> SMGESRVILAFGDSLFAGYGLDKGESYPAKLETALRSHGI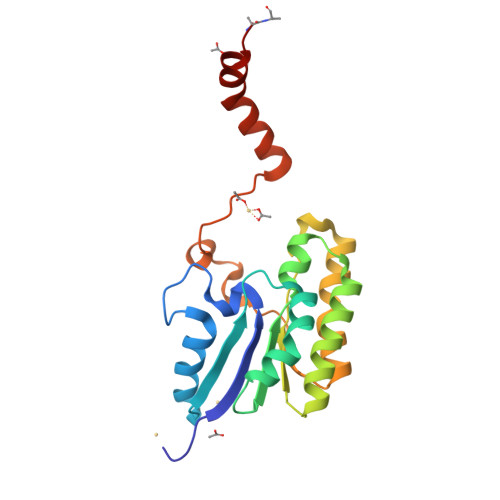NARIINAGVSGDTTAAGLQRIKFVLDSQPDKPELAIVELGGNDLLRGLSPAEARQNLSGILEELQRRKIPILLMGMRAPPNLGAKYQREFDGIYPYLAEKYDAKLVPFFLEAVADRPDLIQKDHVHPTARGVEELVSATSNAVAKALPAKK>[2x]MVTGGGAAPPGTVTEPLPSVIVLSAGRKMAAAAAAASGPGCSSAAGAGAAGVSEWLVLRDGCMHCDADGLHSLSYHPALNAILAVTSRGTIKVIDGTSGATLQASALSAKPGGQVKCQYISAVDKVIFVDDYAVGCRKDLNGILLLDTALQTPVSKQDDVVQLELPVTEAQQLLSACLEKVDISSTEGYDLFITQLKDGLKNTSHETAANHKVAKWATVTFHLPHHVLKSIASAIVNELKKINQNVAALPVASSVMDRLSYLLPSARPELGVGPGRSVDRSLMYSEANRRETFTSWPHVGYRWAQPDPMAQAGFYHQPASSGDDRAMCFTCSVCLVCWEPTDEPWSEHERHSPNCPFVKGEHTQNVPLSVTLATSPAQFPCTDGTDRISCFGSGSCPHFLAAATKRGKICIWDVSKLMKVHLKFEINAYDPAIVQQLILSGDPSSGVDSRRPTLAWLEDSSSCSDIPKLEGDSDDLLEDSDSEEHSRSDSVTGHTSQKEAMEVSLDITALSILQQPEKLQWEIVANVLEDTVKDLEELGANPCLTNSKSEKTKEKHQEQHNIPFPCLLAGGLLTYKSPATSPISSNSHRSLDGLSRTQGESISEQGSTDNESCTNSELNSPLVRRTLPVLLLYSIKESDEKAGKIFSQMNNIMSKSLHDDGFTVPQIIEMELDSQEQLLLQDPPVTYIQQFADAAANLTSPDSEKWNSVFPKPGTLVQCLRLPKFAEEENLCIDSITPCADGIHLLVGLRTCPVESLSAINQVEALNNLNKLNSALCNRRKGELESNLAVVNGANISVIQHESPADVQTPLIIQPEQRNVSGGYLVLYKMNYATRIVTLEEEPIKIQHIKDPQDTITSLILLPPDILDNREDDCEEPIEDMQLTSKNGFEREKTSDISTLGHLVITTQGGYVKILDLSNFEILAKVEPPKKEGTEEQDTFVSVIYCSGTDRLCACTKGGELHFLQIGGTCDDIDEADILVDGSLSKGIEPSSEGSKPLSNPSSPGISGVDLLVDQPFTLEILTSLVELTRFETLTPRFSATVPPCWVEVQQEQQQRRHPQHLHQQHHGDAAQHTRTWKLQTDSNSWDEHVFELVLPKACMVGHVDFKFVLNSNITNIPQIQVTLLKNKAPGLGKVNALNIEVEQNGKPSLVDLNEEMQHMDVEESQCLRLCPFLEDHKEDILCGPVWLASGLDLSGHAGMLTLTSPKLVKGMAGGKYRSFLIHVKAVNERGTEEICNGGMRPVVRLPSLKHQSNKGYSLASLLAKVAAGKEKSSNVKNENTSGTRKSENLRGCDLLQEVSVTIRRFKKTSISKERVQRCAMLQFSEFHEKLVNTLCRKTDDGQITEHAQSLVLDTLCWLAGVHSNGPGSSKEGNENLLSKTRKFLSDIVRVCFFEAGRSIAHKCARFLALCISNGKCDPCQPAFGPVLLKALLDNMSFLPAATTGGSVYWYFVLLNYVKDEDLAGCSTACASLLTAVSRQLQDRLTPMEALLQTRYGLYSSPFDPVLFDLEMSGSSCKNVYNSSIGVQSDEIDLSDVLSGNGKVSSCTAAEGSFTSLTGLLEVEPLHFTCVSTSDGTRIERDDAMSSFGVTPAVGGLSSGTVGEASTALSSAAQVALQSLSHAMASAEQQLQVLQEKQQQLLKLQQQKAKLEAKLHQTTAAAAAAASAVGPVHNSVPSNPVAAPGFFIHPSDVIPPTPKTTPLFMTPPLTPPNEAVSVVINAELAQLFPGSVIDPPAVNLAAHNKNSNKSRMNPLGSGLALAISHASHFLQPPPHQSIIIERMHSGARRFVTLDFGRPILLTDVLIPTCGDLASLSIDIWTLGEEVDGRRLVVATDISTHSLILHDLIPPPVCRFMKITVIGRYGSTNARAKIPLGFYYGHTYILPWESELKLMHDPLKGEGESANQPEIDQHLAMMVALQEDIQCRYNLACHRLETLLQSIDLPPLNSANNAQYFLRKPDKAVEEDSRVFSAYQDCIQLQLQLNLAHNAVQRLKVALGASRKMLSETSNPEDLIQTSSTEQLRTIIRYLLDTLLSLLHASNGHSVPAVLQSTFHAQACEELFKHLCISGTPKIRLHTGLLLVQLCGGERWWGQFLSNVLQELYNSEQLLIFPQDRVFMLLSCIGQRSLSNSGVLESLLNLLDNLLSPLQPQLPMHRRTEGVLDIPMISWVVMLVSRLLDYVATVEDEAAAAKKPLNGNQWSFINNNLHTQSLNRSSKGSSSLDRLYSRKIRKQLVHHKQQLNLLKAKQKALVEQMEKEKIQSNKGSSYKLLVEQAKLKQATSKHFKDLIRLRRTAEWSRSNLDTEVTTAKESPEIEPLPFTLAHERCISVVQKLVLFLLSMDFTCHADLLLFVCKVLARIANATRPTIHLCEIVNEPQLERLLLLLVGTDFNRGDISWGGAWAQYSLTCMLQDILAGELLAPVAAEAMEEGTVGDDVGATAGDSDDSLQQSSVQLLETIDEPLTHDITGAPPLSSLEKDKEIDLELLQDLMEVDIDPLDIDLEKDPLAAKVFKPISSTWYDYWGADYGTYNYNPYIGGLGIPVAKPPANTEKNGSQTVSVSVSQALDARLEVGLEQQAELMLKMMSTLEADSILQALTNTSPTLSQSPTGTDDSLLGGLQAANQTSQLIIQLSSVPMLNVCFNKLFSMLQVHHVQLESLLQLWLTLSLNSSSTGNKENGADIFLYNANRIPVISLNQASITSFLTVLAWYPNTLLRTWCLVLHSLTLMTNMQLNSGSSSAIGTQESTAHLLVSDPNLIHVLVKFLSGTSPHGTNQHSPQVGPTATQAMQEFLTRLQVHLSSTCPQIFSEFLLKLIHILSTERGAFQTGQGPLDAQVKLLEFTLEQNFEVVSVSTISAVIESVTFLVHHYITCSDKVMSRSGSDSSVGARACFGGLFANLIRPGDAKAVCGEMTRDQLMFDLLKLVNILVQLPLSGNREYSARVSVTTNTTDSVSDEEKVSGGKDGNGSSTSVQGSPAYVADLVLANQQIMSQILSALGLCNSSAMAMIIGASGLHLTKHENFHGGLDAISVGDGLFTILTTLSKKASTVHMMLQPILTYMACGYMGRQGSLATCQLSEPLLWFILRVLDTSDALKAFHDMGGVQLICNNMVTSTRAIVNTARSMVSTIMKFLDSGPNKAVDSTLKTRILASEPDNAEGIHNFAPLGTITSSSPTAQPAEVLLQATPPHRRARSAAWSYIFLPEEAWCDLTIHLPAAVLLKEIHIQPHLASLATCPSSVSVEVSADGVNMLPLSTPVVTSGLTYIKIQLVKAEVASAVCLRLHRPRDASTLGLSQIKLLGLTAFGTTSSATVNNPFLPSEDQVSKTSIGWLRLLHHCLTHISDLEGMMASAAAPTANLLQTCAALLMSPYCGMHSPNIEVVLVKIGLQSTRIGLKLIDILLRNCAASGSDPTDLNSPLLFGRLNGLSSDSTIDILYQLGTTQDPGTKDRIQALLKWVSDSARVAAMKRSGRMNYMCPNSSTVEYGLLMPSPSHLHCVAAILWHSYELLVEYDLPALLDQELFELLFNWSMSLPCNMVLKKAVDSLLCSMCHVHPNYFSLLMGWMGITPPPVQCHHRLSMTDDSKKQDLSSSLTDDSKNAQAPLALTESHLATLASSSQSPEAIKQLLDSGLPSLLVRSLASFCFSHISSSESIAQSIDISQDKLRRHHVPQQCNKMPITADLVAPILRFLTEVGNSHIMKDWLGGSEVNPLWTALLFLLCHSGSTSGSHNLGAQQTSARSASLSSAATTGLTTQQRTAIENATVAFFLQCISCHPNNQKLMAQVLCELFQTSPQRGNLPTSGNISGFIRRLFLQLMLEDEKVTMFLQSPCPLYKGRINATSHVIQHPMYGAGHKFRTLHLPVSTTLSDVLDRVSDTPSITAKLISEQKDDKEKKNHEEKEKVKAE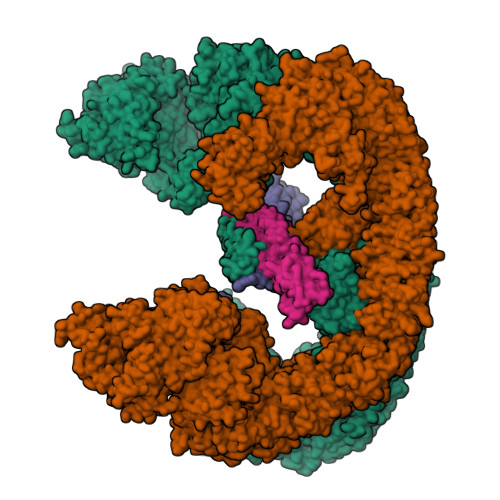NGFQDNYSVVVASGLKSQSKRAVSATPPRPPSRRGRTIPDKIGSTSGAEAANKIITVPVFHLFHKLLAGQPLPAEMTLAQLLTLLYDRKLPQGYRSIDLTVKLGSRVITDPSLSKTDSYKRLHPEKDHGDLLASCPEDEALTPGDECMDGILDESLLETCPIQSPLQVFAGMGGLALIAERLPMLYPEVIQQVSAPVVTSTTQEKPKDSDQFEWVTIEQSGELVYEAPETVAAEPPPIKSAVQTMSPIPAHSLAAFGLFLRLPGYAEVLLKERKHAQCLLRLVLGVTDDGEGSHILQSPSANVLPTLPFHVLRSLFSTTPLTTDDGVLLRRMALEIGALHLILVCLSALSHHSPRVPNSSVNQTEPQVSSSHNPTSTEEQQLYWAKGTGFGTGSTASGWDVEQALTKQRLEEEHVTCLLQVLASYINPVSSAVNGEAQSSHETRGQNSNALPSVLLELLSQSCLIPAMSSYLRNDSVLDMARHVPLYRALLELLRAIASCAAMVPLLLPLSTENGEEEEEQSECQTSVGTLLAKMKTCVDTYTNRLRSKRENVKTGVKPDASDQEPEGLTLLVPDIQKTAEIVYAATTSLRQANQEKKLGEYSKKAAMKPKPLSVLKSLEEKYVAVMKKLQFDTFEMVSEDEDGKLGFKVNYHYMSQVKNANDANSAARARRLAQEAVTLSTSLPLSSSSSVFVRCDEERLDIMKVLITGPADTPYANGCFEFDVYFPQDYPSSPPLVNLETTGGHSVRFNPNLYNDGKVCLSILNTWHGRPEEKWNPQTSSFLQVLVSVQSLILVAEPYFNEPGYERSRGTPSGTQSSREYDGNIRQATVKWAMLEQIRNPSPCFKEVIHKHFYLKRVEIMAQCEEWIADIQQYSSDKRVGRTMSHHAAALKRHTAQLREELLKLPCPEGLDPDTDDAPEVCRATTGAEETLMHDQVKPSSSKELPSDFQLSAWSHPQFEK;>[2x]AVPIAQKSEPHSLSSEALMRRAVSLVTDSTSTFLSQTTYALIEAITEYTKAVYTLTSLYRQYTSLLGKMNSEEEDEVWQVIIGARAEMTSKHQEYLKLETTWMTAVGLSEMAAEAAYQTGADQASITARNHIQLVKLQVEEVHQLSRKAETKLAEAQIEELRQKTQEEGEERAESEQEAYLRED>[2x]MTNIFTPIEEALEAYKNGEFLIVMDDEDRENEGDLIMAAELITQEKMAFLVRYSSGYVCVPLSEERA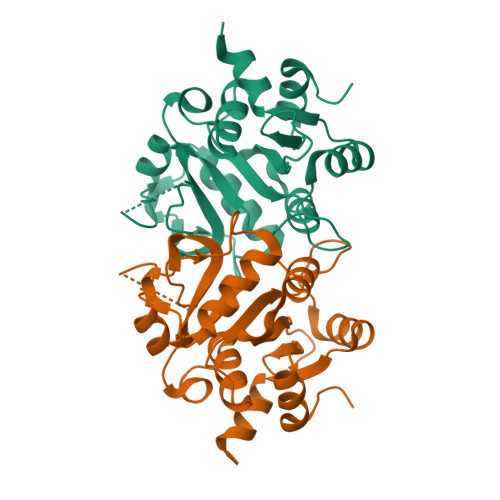NQLELPPMLANRSDRHGTAYTITCDFAEGTTTGISAHDRALTTRSLANPNSKPQDFIKPGHILPLRAVPGLLKKRRGHTEAAVQLSTLAGLQPAGVICELVRDEDGLMMRLDDCIQFGKKHGIKIININQLVEYISK> MDETVAEFIKRTILKIPMNELTTILKAWDFLSENQLQTVNFRQRKESVVQHLIHLCEEKRASISDAALLDIIYMQFHQHQKVWEVFQMSKGPGEDVDLFDMKQFKNSFKKILQRALKNVTVSFRETEENAVWIRIAWGTQYTKPNQYKPTYVVYYSQTPYAFTSSSMLRRNTPLLGQALTIASKHHQIVKMDLRSRYLDSLKAIVFKQYNQTFETHNSTTPLQERSLGLDINMDSRIIHENIVEKERVQRITQETFGDYPQPQLEFAQYKLETKFK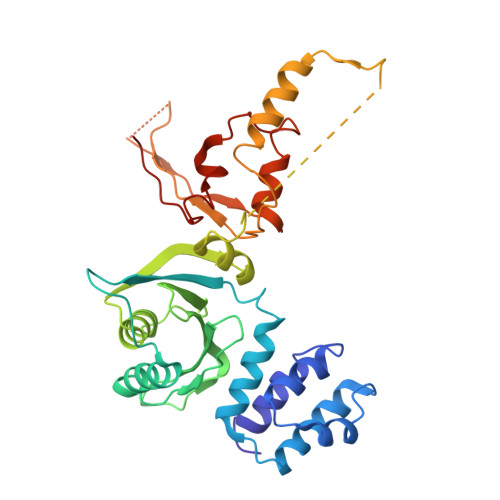SGLNGSILAEREEPLRCLIKFSSPHLLEALKSLAPAGIADAPLSPLLTCIPNKRMNYFKIRDKHHHHHH> MLEAKFEEASLFKRIIDGFKD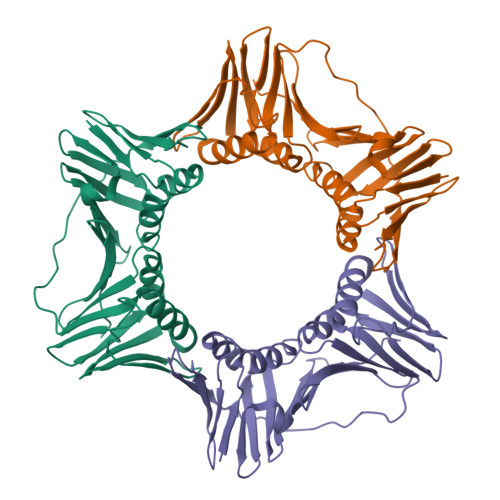CVQLVNFQCKEDGIIAQAVDDSRVLLVSLEIGVEAFQEYRCDHPVTLGMDLTSLSKILRCGNNTDTLTLIADNTPDSIILLFEDTKKDRIAGYSLKLMDIDADFLKIEELQYDSTLSLPSSEFSKIVRDLSQLSDSINIMITKETIKFVADGDIGSGSVIIKPFVDMEHPETSIKLEMDQPVDLTFGAKYLLDIIKGSSLSDRVGIRLSSEAPALFQFDLKSGFLQFFLAPKFNDEE> MTKTPEAPVPRTMEKDHTQQINVIIVGLGIAGLTAAIECHRKGHKVIAFEKTPKMMHIGDIFSIGPNAESVIRQWKDGAISRALNEARCAIDEIKVFDETGKLQNVNTMEGYREGEGYVINRAEAVDIFFEYAQSLGIDIRFNSNVTEYWET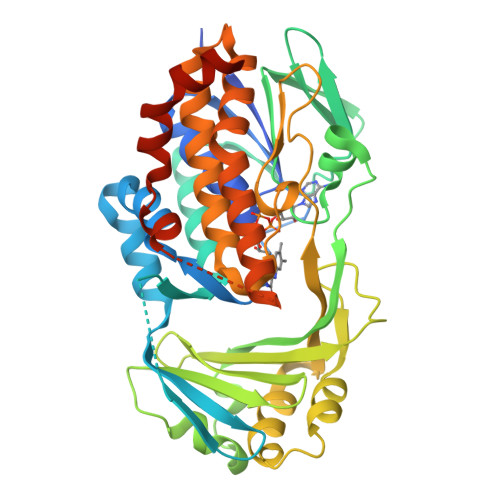PHNAGIIVDGLKIEADCVIATDGIHSKARNAICGAVVQPKKTGSAIYRSGYAMEELRGHSGAVWLTEGKEDVDQLYHFIGKDITVLVGTGRRGKDVYWGCMHKSLHDVSESWIQVSDVRRAIELISDWNVRDRLEPIMACTPQGKCFDHLVMTMDQLPSWVSPKHRMIVLGDAAHPFLPNTGQGANQAIEDGATVAICLELAGKNQVTKGVQVAERLRYQRVAKIQELGHRMLKTLQNADWDGEKDEDAPTMITRPAWIYSHDCQQYAYNEFQTVAQLVSERRDFHHHHHH>MEEECRVLSIQSHVVRGYVGNRAATFPLQVLGFEVDAVNSVQFSNHTGYSHWKGQVLNSDELQELYDGLKLNHVNQYDYVLTGYTRDKSFLAMVVDIVQELKQQNPRLVYVCDPVMGDQRNGEGAMYVPDDLLPVYREKVVPVADIITPNQFEAELLTGRKIHSQEEALEVMDMLHSMGPDTVVITSSNLLSPRGSDYLMALGSQRTRAPDGSVVTQRIRMEMHKVDAVFVGTGDLFAAMLLAWTHKHPNNLKV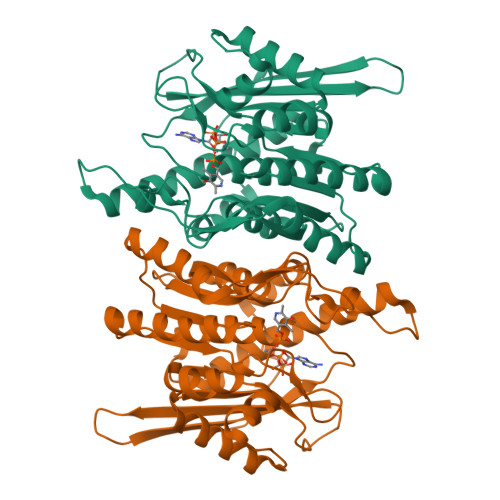ACEKTVSAMHHVLQRTIKCAKAKSGEGVKPSPAQLELRMVQSKKDIESPEIVVQATVL[8x]> TKRLIHENQGQCCGLIDLMREYQNLKSAVSKVLENASSVIVTRTTIKDQEDLKWAFSKHETAKNKMNYKQKDLDNFTSKGKHLLSELKKIHSSDFSLVKTDMESTVDKWLDVSEKLEENMD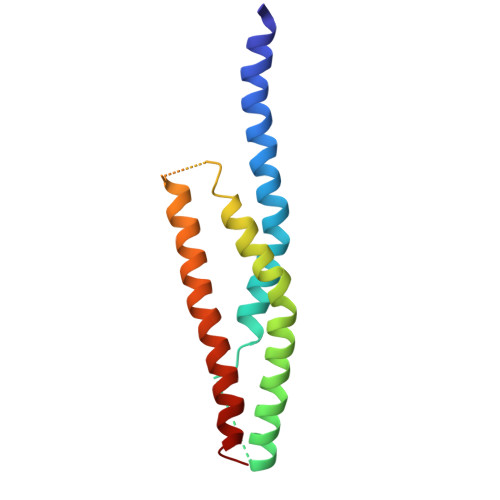RLRVSLSIWD>M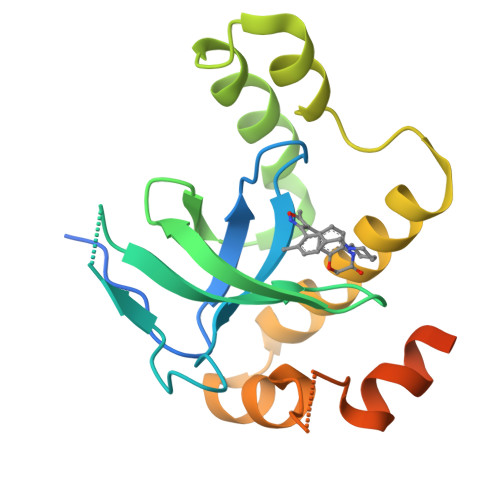GGGPNTGRDKDHLLKYNVGDLVWSKVSGYPWWPCMVSADPLLHSYTKLKGQAASARQYHVQFFGDAPERAWIFEKSLVAFEGEGQFEKLCQESAKQAPTAAEKIKLLAPISGKLRAQWEMGIVQAEEAASMSVEERKAKFTFLYVGDQLHLNPQVAKEAGIAAEGGGENLYFQGSHHHHHH[2x]> MLAKRIIACLDVKDGRVVKGTNFENLRDSGDPVELGKFYSEIGIDELVFLDITASVEKRKTMLELVEK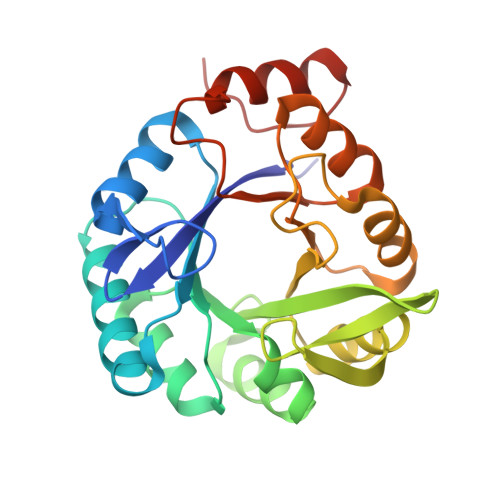VAEQIDIPFTVGGGIHDFETASELILRGADKVSINTAAVENPSLITQIAQTFGSQAVVVAIDAKRVDGEFMVFTYSGKKNTGILLRDWVVEVEKRGAGEILLTSIDRDGTKSGYDTEMIRFVRPLTTLPIIASGGAGKMEHFLEAFLAGADAALAASVFHFREIDVRELKEYLKKHGVNVRLEGL> DKLTQQDYNTDFIYESHHRQPKESLTHASVLSAYTASYKTTAIKSIADNAVVLDIGYGKGNDGPRYAVRPLTVTGIDTAARMLAIADQNKPENVTLVKQGFFTHITKTSNTYTHVIAFNSLHYPLASSHPDTLVQRLPTCPANILIPCHHLLEGIQTPTYSVVKDEDMWCVKVTKNEFIESSYNYDVFVKALESKYHVTIGSLLDCVEKPSTRSITPTLWTAMRNFVNNDQEMQRILSGYITFNLTPLPPKVEIINDWLD

Interestingly however, we and others have identified a putative N7-MTase in pp1a (N7-MT-1a) of several members of the large-genome Tobaniviridae family. Here, we confirmed the presence of a Class-1, N7-specific MTase in pp1a of WBV, a member of the Tobaniviridae family. The WBV N7-MT-1a exhibits a canonical RF βαβ structural motif, similar to that of diverse N7-MTases, including that of E. cuniculi, humans and two large dsDNA viruses, despite low sequence similarity. The WBV MTase is therefore RNA Cap-guanine specific, with a strong preference for methylation of an open (GpppN) cap structure.

A C-terminally truncated construct (Asp1374–Asp1633, WBV-260) yielded a clean product of expected molecular weight, possessing activity levels equivalent to WBV-295. The WBV-260 protein crystallized in two different space groups, C2 and P21, with one monomer per asymmetric unit, diffracting to 2.6 and 1.7 Å, respectively. We present its crystal structure at 1.7 Å resolution, revealing that it adopts a canonical RF secondary structure. The two structures are almost identical, with the exception of the last flexible C-terminal helix that is not visible in the Tantalum-soaked crystal. AdoHcy, the by-product of the methylation reaction, is found in the active-site of both structures. The central core of the WBV N7-MT-1a adopts a canonical Rossmann-fold (RF), with an alternating βαβ structural motif, characteristic of the class I family of MTases. This core structure is formed by a central, seven-stranded β-sheet (ordered β3, β2, β1, β4, β5, β10, β9), flanked by α-helices on each side (α1, α2, α3 on one side, and α4, α5/α6 and α7 on the other). In addition to this central fold, two other structural features are present; a flexible ‘3β-flap’ domain comprised of a short α-helical loop followed by three anti-parallel β-strands (β1 and β6–β8) and an α-helical bundle (β2, α8 and α9) wrapping around α1, herein referred to as the α-bundle region. The first 22 residues of the WBV N7-MT-1a are unresolved in the structure. As with other, class I MTases, AdoHcy binds in a deep, predominantly negatively charged groove, formed by the loops between β1–α2, β2–α3, β3–α4 and β4–α5. The AdoHcy adopts an anti- conformation, similar to that seen in the Ecm1, Hmc1 and ASFV MTase structures.7-(furan-2-yl)-2-hydroxyisoquinoline-1,3(2H,4H)-dione 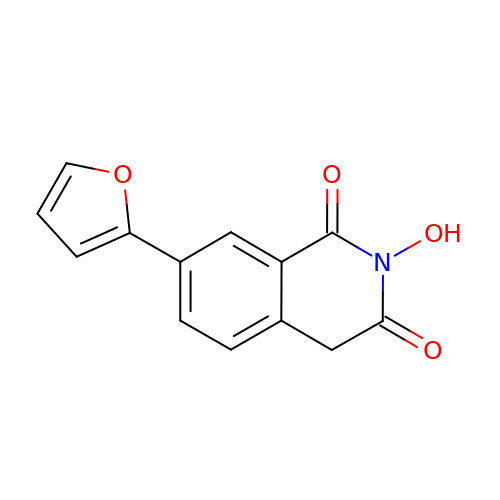| C13 H9 N O4 | FMBJYDTZYGCAIN-UHFFFAOYSA-N> MKESVRFLTDFGEISDAISDLLTSSPNFNVISAIGPQGAGKSTLLSMLAGNNSRQMYREYVFRPVSREANEQSRHQTIQIDIYIVNHQIFLDCQPMYSFSIMEGLPKVRGGRFDDSTAMSDTLRLTAFLLYVSHTVLVVSETHYDKVIIDTLRVAEQIRPYLAIFRPKLAIDRKTNLVFIKTKASSIDLAPTVIREREELLRLSFQDS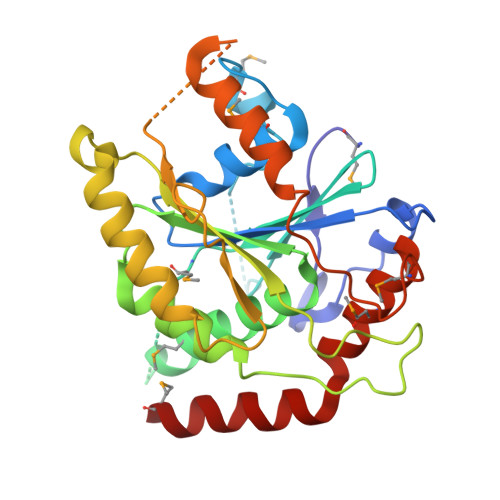RWLKVSQEPFKTLIVLEEIRVRREHLFEEGDEPDEAASLNEFDEQIAELREELQKNREDFTVETAAMDEKKWLDMCREVIRDKTLHKTLKEYQRAMT> EQTSIAHLTSDDVNLPGSDFFRFYRSADKQEKEKARIYLLGVLDATEGKSWCQYSQLQTVTLQEFVFEFFNKLPAARLHERAAPLIEEALATRFPCKGGKA;> MKPLYRQLKSSHYSSDYSSPGYLAAEAVYAEIGYELDTLLKQNPGYANTCAVRMSLALLKTGISFKGRLPIKKGAYKGKTIEPGAKLLADQLHRSSSFGKAKIFFNAPDAEKGIGNKKGVVFFNKITNYDGGHIDLIEPENSLLTCHSHCYFNCKEVWFWELS

Some Gram-negative bacteria target their competitors by exploiting the type VI secretion system to extrude toxic effector proteins. To prevent self-harm, these bacteria also produce highly specific immunity proteins that neutralize these antagonistic effectors. The opportunistic pathogen Serratia marcescens has recently been shown to utilize T6-dependent secretion of two family 4 amidases, Ssp1 and Ssp2, to mediate antibacterial activity. In S. marcescens, the resistance-associated proteins Rap1a and Rap2a neutralize Ssp1 and Ssp2, respectively.

Following purification using a co-expression strategy, we determined the structure of the Ssp1–Rap1a complex at about 2.0 Å resolution. The structure of the Ssp1–Rap1a complex revealed a tightly bound heteromeric assembly with two effector molecules flanking a Rap1a dimer. The overall dimensions of this heteromeric assembly are about 90 × 50 × 50 Å and its molecular weight is approximately 60 kDa, consistent with that observed by size-exclusion chromatography during purification of the complex. The model contains residues 1–163 of Ssp1 and residues 30–123 of Rap1a. The solvent-accessible surface area of Ssp1 is 5840 Å2 and about 16% of this (960 Å2) is occluded when the complex with Rap1a is formed. Rap1a interacts with Ssp1 using residues in α1, α3, α4, α5 and the α4–α5 loop. In particular, the α4–α5 loop and α4 of Rap1a are directly positioned to block the Ssp1 active site. Arg119, Arg66, Lys59, Glu94 and Glu94 of Rap1a form salt-bridge interactions with Asp37, Asp16, Glu140, Arg53 and Arg53 of Ssp1, respectively. In the α1–α2 loop of Ssp1, Tyr17 is relocated by about 7 Å to interact with Tyr50 and Arg62 of Rap1a. Rap1a, which has a completely different fold to the conventional Tai4 proteins, does not possess a protruding loop, but in the complex a helix is positioned to block the effector active site and the interactions that stabilize the complex involve residues in the C-terminal subdomain of the effector rather than the N-terminal subdomain.>[2x]SLLKLAIPKGRLEEKVMTYLKKTGVIFERESSILREGKDIVCFMVRPFDVPTYLVHGVADIGFCGTDVLLEKETSLIQPFFIPTNISRMVLAGPKGRGIPEG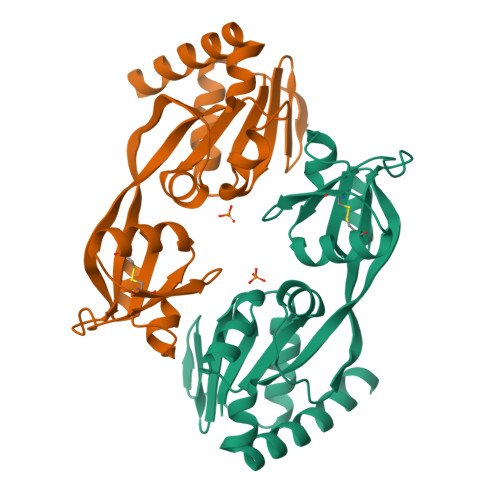EKRIATKFPNVTQRYCESKGWHCRIIPLKGSVELAPIAGLSDLIVDITETGRTLKENNLEILDEIFVIRTHVVVNPVSYRTKREEVVSFLEKLQEVIEHDSNEQSRGEGGSHHHHHH P1-(ADENOSINE-5'-P5-(URIDINE-5')PENTAPHOSPHATE | C19 H28 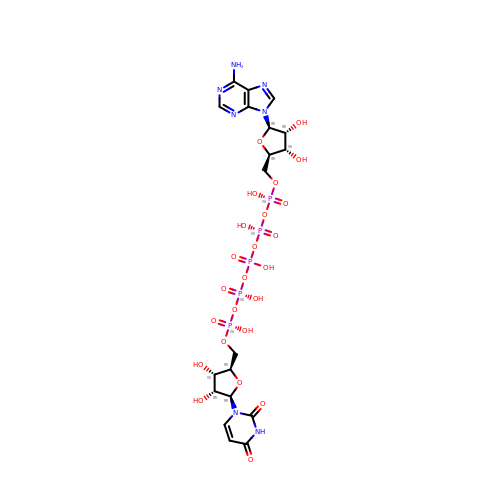N7 O24 P5 | CPTLFMDLEWCNMJ-KPKSGTNCSA-N> RVADTVGTGPTNSEAIPALTAAETGHTSQVVPGDTMQTRHVKNYHSRSESTIENFLCRS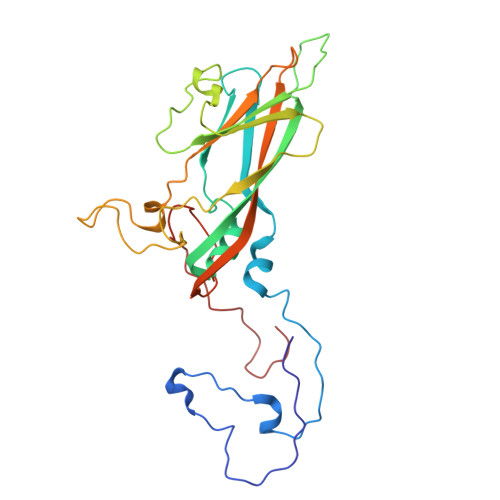ACVYFTEYENSGAKRYAEWVLTPRQAAQLRRKLEFFTYVRFDLELTFVITSTQQPSTTQNQDAQILTHQIMYVPPGGPVPDKVDSYVWQTSTNPSVFWTEGNAPPRMSIPFLSIGNAYSNFYDGWSEFSRNGVYGINTLNNMGTLYARHVNAGSTGPIKSTIRIYFKPKHVKAWIPRPPRLCQYEKAKNVNFQPSGVTTTRQSITTMTN The tandem-repeat galectins, of which galectin-4 is a member, contain two distinct CRDs at their N- and C-termini, connected by a variable-length linker region that is susceptible to proteolytic degradation. The overall fold of human galectin-4N is the conserved galectin β-sandwich fold comprising two β-sheets, F1–F5 and S1–S6, of which the concave side of the β-sandwich (S1–S6) contains the saccharide-binding site. As with other galectin CRDs, the amino acids forming the binding sub-sites C and D are conserved, while those that construct the A, B and E sub-sites are slightly different, granting galectin-4N its unique binding specificity. To investigate the interaction between human galectin-4N and its natural saccharide ligands, we have determined the crystal structures of human galectin-4N in complex with glycerol (the cryoprotectant), lactose, lactose-3′-sulfate (3′SuL), and 2′-fucosyllactose (2′FL) at 1.70–2.00 Å resolution.

The galectin-4N-lactose complex structure was determined at 1.90 Å resolution from crystals grown in a PEG-based condition that is different to the other crystals reported here (which were crystallised in high concentration of sodium formate). The binding sites of all 4 monomers within the asymmetric unit contained unambiguous density for the lactose molecule. However, due to the presence of calcium acetate in the crystallisation condition of the galectin-4N-lactose complex, the four galectin-4N monomers each contained a bound Ca2+ ion, coordinated by the backbone carbonyls of Phe68 and Gly70, the carboxylate of Asp72 and 3 water molecules. The binding interactions observed between galectin-4N and lactose are the same as the conserved interactions observed in previously reported galectin-lactose complex structures. The C4′ hydroxyl of the galactose saccharide interacts with His63, Asn65 and Arg67. The C6′ hydroxyl of the galactose residue interacts with Asn77 and Glu87. The C3 hydroxyl of the glucose residue is in interaction distance of Arg67, Glu87 and Arg89. Additionally, the C2 hydroxyl of glucose is in hydrogen bonding distance of Arg89. Within the asymmetric unit, Arg89 interacts with lactose only in monomer A, but instead forms crystallographic salt bridges with Asp55 of other monomers in monomers B, C and D. As we observed in the interactions between the galectin-3 Arg186 (equivalent to galectin-4N Arg89) and other saccharide ligands, the galectin-4N Arg89 interaction with lactose and similar ligands may be transient. The presence of galectin-4N Arg89 which can form transient interactions with the lactose C2 and C3 hydroxyls could contribute to the slightly higher affinity, as the galectin-4C equivalent at this position is Lys261, which does not form similar interactions.

>[4x]MAYVPAPGYQPTYNPTLPYYQPIPGGLNVGMSVYIQGVASEHMKRFFVNFVVGQDPGSDVAFHFNPRFDGWDKVVFNTLQGGKWGSEERKRSMPFKKGAAFELVFIVLAEHYKVVVNGNPFYEYGHRLPLQMVTHLQVDGDLQLQSINFIGGQPL> MTSPAKFKKDKEIIAEYDTQVKEIRAQLTEQMKCLDQQCELRVQLLQDLQDF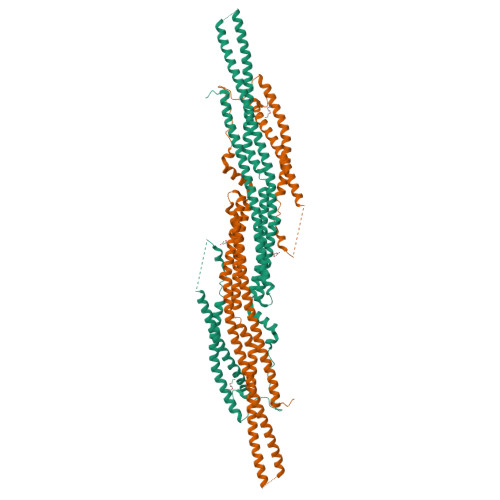FRKKAEIEMDYSRNLEKLAERFLAKTRSTKDQQFKKDQNVLSPVNCWNLLLNQVKRESRDHTTLSDIYLNNIIPRFVQVSEDSGRLFKKSKEVGQQLQDDLMKVLNELYSVMKTYHMYNADSISAQSKLKEAEKQEEKQIGKSVKQEDRQTPRSPDSTANVRIEEKHVRRSSVKKIEKMKEKRQAKYTENKLKAIKARNEYLLALEATNASVFKYYIHDLSDLIDQCYDLGYHASLNRALRTFLSAELNLEQSKHEGLDAIENAVENLDATSDKQRLMEMYNNVFCPPMKFEFQPHMGDMASQLCAQQPVQSELVQRCQQLQSRLSTLKIENEEVKKTMEATLQTIQDIVTVEDFDVSDCFQYSNSMESVKSTVSETFMSKPSIAKRRANQQETEQFYFTKMKEYLEGRNLITKLQAKHDLLQKTLGESQRT> MAYRKRGARRETNLKQDDRMQEKEENKNVNTNSENKNATKPQLSEKVLSQKEEVITDNQEEIKIADEVKKSNKEESKQLLEVLKTKEEHQKEVQYEILQKTIPTFEPKESILKKLEDIKPEQVKKQTKLFRIFEPRQLPVYRANGEKELRNRWYWKLKRDTLPDGDYDVREYFLNLYDQVLTEMPDYLLLKDMAVENKNSRDAGKVVDSETAAICDAIFQDEETEGVVRRFIAEMRQRVQADRNVVNYPSILHPIDHAFNEYFLQHQLVEPLNNDIIFNYIPERIRNDVNYILNMDRNLPSTARYIRPNLLQDRLNLHDNFESLWDTITTSNYILARSVVPDLKELVSTEAQIQKMSQDLQLEALTIQSETQFLTGINSQAANDCFKTLIAAMLS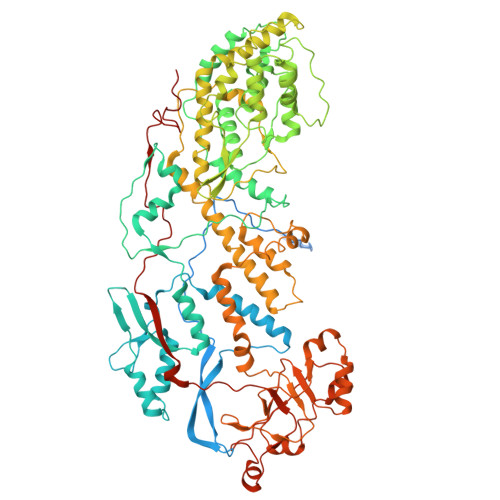QRTMSLDFVTTNYMSLISGMWLLTVVPNDMFIRESLVACQLAIINTIIYPAFGMQRMHYRNGDPQTPFQIAEQQIQNFQVANWLHFVNNNQFRQVVIDGVLNQVLNDNIRNGHVVNQLMEALMQLSRQQFPTMPVDYKRSIQRGILLLSNRLGQLVDLTRLLAYNYETLMACITMNMQHVQTLTTEKLQLTSVTSLCMLIGNATVIPSPQTLFHYYNVNVNFHSNYNERINDAVAIITAANRLNLYQKKMKSIVEDFLKRLQIFDISRVPDDQMYRLRDRLRLLPVEIRRLDIFNLILMNMEQIERASDKIAQGVIIAYRDMQLERDEMYGYVNIARNLDGFQQINLEELMRTGDYAQITNMLLNNQPVALVGALPFITDSSVISLVAKLDATVFAQIVKLRKVDTLKPILYKINSDSNDFYLVANYDWVPTSTTKVYKQIPQQFDFRASMHMLTSNLTFTVYSDLLAFVSADTVEPINAVAFDNMRIMNEL>MGSSHHHHHHSSGLVPRGSGGYEIPARLRTLHNLVIQYASQGRYEVAVPLCKQALEDLEKTSGHDHPDVATMLNILALVYRDQNKYKDAAHLLNDALAIREKTLGKDHPAVAATLNNLAVLYGKRGKYKEAEPLCKRALEIREKVLGKFHPDVAKQLSNLALLCQNQGKAEEVEYYYRRALEIYATRLGPDDPNVAKTKNNLASCYLKQGKYQDAETLYKEILTRAHEKEFGSVNGENKPIWMHAEEREESKDKRRDSAPYGEYGSWYKACKVDSPTVNTTLRSLGALYRRQGKLEAAHTLEDCASRSRKQGLD[3x]

Kinesin1 functions as a hetero-tetramer composed of a dimer of kinesin heavy chains (KHC) bound to two kinesin light chains (KLC). KLC is also composed of three regions: a N-terminal Heptad Repeat (HR) region that binds to the KHC stalk, a TPR (Tetratrico Peptide Repeat) domain involved in cargo recruitment, and a variable C-terminal region. The TPR domain of KLC1/2 belongs to the 42PR motif family and consists of six TPR motifs (TPR1-6) with a non-TPR region of 40 residues inserted between TPR5 and TPR6 motifs. The N-terminal capping A1 helix exhibits structural plasticity adopting two distinct and defined orientations relative to the rest of the TPR domain.

In order to analyse the structural impact of LFP-motif binding on the TPR domain of KLC, especially at the TPR1 motif, we crystallized an unbound complete TPR domain of KLC2 and compared it to the previously solved KLC2-TPR bound to LFP-motif. The structure of KLC2-TPR[A1-B6] adopts the common KLC-TPR structural fold composed of 12 α-helices (namely A1 to B6 helices). The non-TPR region of 40 residues connecting the TPR5 motif to the TPR6 motif is made up of an α-helix (αn1; residue 410–420), followed by a disordered region (421–444) that is not modeled in the crystal structure due to the absence of electron density. Interestingly, the three KLC2-TPR[A1-B6] molecules make the same crystal packing contact with a 2-fold axis symmetrical counterpart leading to TPR1:TPR1’ interactions. The two anti-parallel A1/B1 helices from each molecule are roughly perpendicular to each other and bury a total surface area of 1533 Å2 involving numerous hydrophobic residues. SEC-MALLS experiment reveals that KLC2-TPR[A1-B6] is a monomer in solution with a weight-averaged mass of 36.5 ± 1.0 kDa. Thus, this TPR1:TPR1’ contact alone is not sufficient to stabilize such a dimer in solution. In the KLC2-TPR[A1-B6] structure (this study) which is the unique unbound form, the A1 helix exhibits a “IN” orientation, while in the three ligand-bound forms, the A1 helix exhibits one or the other orientation. Finally, because of the crystal packing contacts at the TPR1 motif, we cannot elucidate what component of the crystal packing contacts or the binding of the LFP-motif triggers the A1 helix reorientation observed in KLC2-TPR[A1-B6] (this study) structure.> MAHHHHHHMQQIQRDIAQALQVQPPF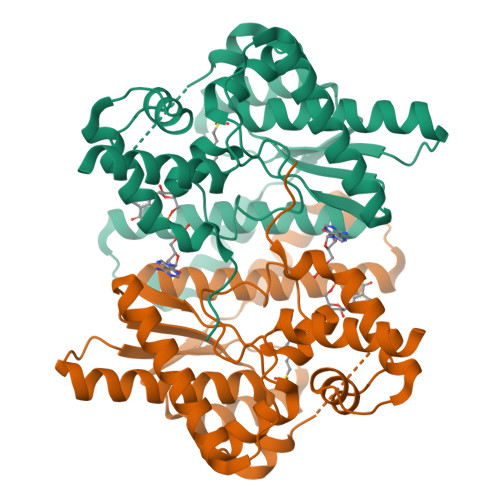QSEADVQAQIARRIAFIQQCLKDSGLKTLVLGISGGVDSLTAGLLAQRAVEQLREQTGDQAYRFIAVRLPYQVQQDEADAQASLATIRADEEQTVNIGPSVKALAEQLEALEGLEPAKSDFVIGNIKARIRMVAQYAIAGARGGLVIGTDHAAEAVMGFFTKFGDGACDLAPLSGLAKHQVRALARALGAPENLVEKIPTADLEDLRPGHPDEASHGVTYAEIDAFLHGQPLREEAARVIVDTYHKTQHKRELPKAP> ASPQRGRPRLNAARTTFVGDNGQPLRGPYTSTEWTAAAPYDQIARVKELGFNAVHLYAECFDPRYPAPGSKAPGYAVNEIDKIVERTRELGLYLVITIGNGANNGNHNAQWARDFWKFYAPRYAKETHVLYEIHNEPVAWGPPYSSSTANPPGAVDMEIDVYRIIRTYAPETPVLLFSYAVFGGKGGAAEALKDIRAFNKAVFGNENAVWTNEAVAFHGYAGWQETTIAVEELLKAGYPCFMTEYAGGAWGSGMGGLDVELTYELERLGVSWLTFQYIPPTGVSDDVTKPEYFSALVENSGLSWTPDYGNWPAARGVYGNGGLARETATWINNFLTGTTRIEAEDFDWGGNGVSYYDTDSV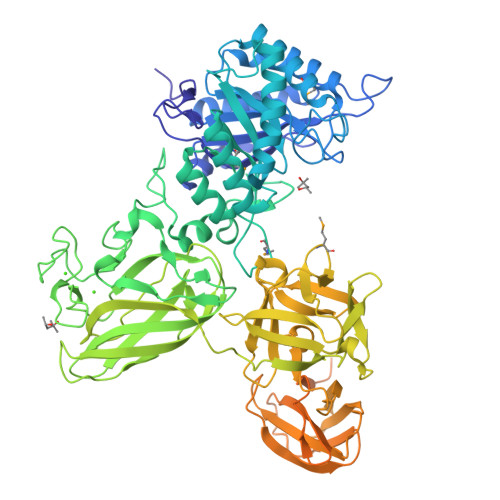NVGGQYRPDEGVDIEKTSDTGGGYNVGWISEGEWLEYTIRVRNPGYYNLSLRVAGISGSRVQVSFGNQDKTGVWELPATGGFQTWTTATRQVFLGAGLQKLRINALSGGFNLNWIELSPISTGTIPDGTYKFLNRANGKTLQEVTGNNSIITADYKGITEQHWKIQHIGGGQYRISSAGRGWNWNWWMGFGTVGWWGTGSSTCFIISPTGDGYYRIVLVGDGTNLQISSGDPSKIEGKAFHGGANQQWAILPVSAPAFPTGLSAVLDSSGNTANLTWNAAPGANSYNVKRSTKSGGPYTTIATNITSTNYTDTGVATGTKYYYVVSAVSNGVETLNSAEAILQYPKLTGTVIGTQGSWNNIGNTIHKAFDGDLNTFFDGPTANGCWLGLDFGEGVRNVITQIKFCPRSGYEQRMIGGIFQGANKEDFSDAVTLFTITSLPGSGTLTSVDVDNPTGFRYVRYLSPDGSNGNIAELQFFGTPAGEENDDVHLGDILEHHHHHH The discovery of the founding member of the LanM family of lanthanide-binding proteins demonstrated that nature has evolved macromolecules surpassing the selectivity of synthetic f-element chelators. The natural lanthanide-binding protein lanmodulin (LanM)4,5 is a sustainable alternative to conventional solvent-extraction-based separation. First, LanMs possess four EF-hand motifs. Second, adjacent EF hands in LanMs are separated by 12–13 residues—rather than the typical ≈25 residues in CaII-responsive EF-hand proteins—resulting in an unusual three-helix bundle architecture with the metal-binding sites on the periphery.

To understand the basis for LRE versus HRE discrimination, we also determined a 1.4-Å-resolution structure of DyIII–Hans-LanM. The structure of DyIII–Hans-LanM confirms the importance of second-sphere control of ligand positioning. In EF3, this carboxylate shift lengthens the distance between Arg100 and the proximal Oε of Glu91 from 2.9 Å (in LaIII–Hans-LanM) to 3.2 Å. The rearrangement of this second-sphere hydrogen-bonding network suggests a structural basis for RE-dependent differences in Kdimer values. By contrast, even though DyIII induces the same overall response as LaIII in stoichiometric titrations, in the chelator-buffered DyIII titrations Hans-LanM exhibits a lesser conformational response (1.8-fold increase). The main response to DyIII occurs at 2.6 nM, >30-fold higher than with the LREs, and with little or no cooperativity (n = 1.3). The apoprotein and DyIII-bound protein weakly dimerize, with Kdimer values of 117 µM and 60 µM, respectively, consistent with the ratios of monomer and dimer reflected in the SEC and MALS traces. Thus, LaIII favours Hans-LanM’s dimerization by >100-fold over DyIII.

>ASGADALKALNKDNDDSLEIAEVIHAGATTFTAINPDGDTTLESGETKGRLTEKDWARANKDGDQTLEMDEWLKILRTRFKRADANKDGKLTAAELDSKAGQGVLVMIMK[4x]>[2x]SDLPRHIAVLCDGNRRWARSAGYDDVSYGYRMGAAKIAEMLRWCHEAG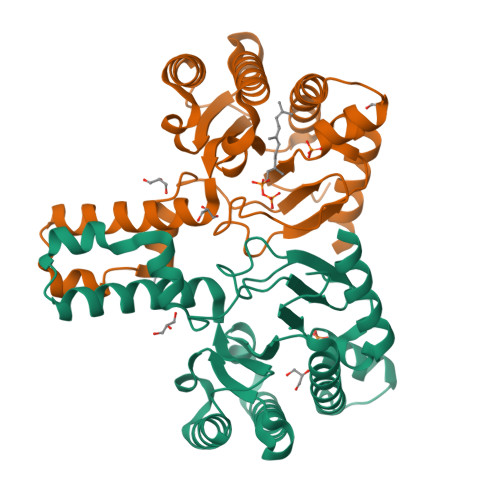IELATVYLLSTENLQRDPDELAALIEIITDVVEEICAPANHWSVRTVGDLGLIGEEPARRLRGAVESTPEVASFHVNVAVGYGGRREIVDAVRALLSKELANGATAEELVDAVTVEGISENLYTSGQPDPDLVIRTSGEQRLSGFLLWQSAYSEMWFTEAHWPAFRHVDFLRALRDYSAR> YAIAGNGVRVTYDADGQTITLYRTEGSGLIQMSKPSPLGGPVVGGQEVQDFSHISCDVEQSTSGVMGSGQRMTITSQSMSTGLIRTYVLETSDIEEGVVYTATSYEAGASDVEVSWFIGSVYELYGAEDRIWSYNGGGEGPMHYYDTLQKIDLTDSGKFSRENKQDDTAASIPVSDIYIADGGITVGDASATRREVHTPVQETSDSAQVSIGWPGKVIAAGSVIEIGESFAVVHPGDYYNGLRGYKNAMDHLGVIMPAPGDIPDSSYDLRWESWGWGFNWTIDLIIGKLDELQAAGVKQITLDDGWYTNAGDWALNPEKFPNGASDALRLTDAIHEHGMTALLWWRPCDGGIDSILYQQHPEYFVMDADGRPARLPTPGGGTNPSLGYALCPMADGAIASQVDFVNRAMNDWGFDGFKGDYVWSMPECYNPAHNHASPEESTEKQSEIYRVSYEAMVANDPNVFNLLCNCGTPQDYYSLPYMTQIATADPTSVDQTRRRVKAYKALMGDYFPVTADHNNIWYLSAVGTGSVLIEKRDLSGTAKEEYEKWLGIADTVQLQKGRFIGDLYSYGFDPYETYVVEKDGVMYYAFYKDGSKYSPTGYPDIELKGLDPNKMYRIVDYVNDRVVATNLMGDNAVFNTRFSDYLLVKAVEISEPDP

Recent studies identified two synergistic enzymes from Flavonifractor plautii, namely, N-acetylgalactosamine deacetylase (FpGalNAcDeAc) and galactosaminidase (FpGalNase), which efficiently convert A-type RBCs to O-type by removing A antigens. In this study, we investigated two enzymes from Flavonifractor plautii, N-acetylgalactosamine deacetylase (FpGalNAcDeAc) and galactosaminidase (FpGalNase), which demonstrate synergistic activity in efficiently converting A-type RBCs to O-type. O-type RBCs lack immunodominant sugars found in A (α-N-acetylgalactosamine) and B antigen (galactose), making them essential in emergencies and when matching blood types is not feasible. One promising solution is the enzymatic conversion of all red blood cell (RBC) types into universal O-type RBCs.

We successfully determined the cryo-electron microscopy (cryo-EM) structure of full-length FpGalNase at 2.56 Å resolution. The N-terminal region (residue 27–699) adopts a disc-like conformation divided into three segments: the N-domain, the central GH36 domain, and the C-domain. Structural similarity analysis using the Dali tool revealed that each domain exhibits a structure similar to α-galactosidase, despite low sequence identity. Conserved residues in FpGalNase active site include W317, D346, D347, W387, K461, and D463 (patch A), along with specific non-conserved residues (Y464, C513, and D532) in patch B, which afford a more open catalytic center conformation and may determine its substrate specificity. Site-directed mutagenesis of D463A, Y464A, C513A, and D532A confirmed the functional importance of these residues, as mutations led to significant reductions in conversion activity, with D463A, C513A, and D532A nearly inactive, and the mutants were unable to convert A-type RBCs to O-type in samples from healthy donors. Moreover, comparison between the experimental structure and the AlphaFold-predicted structure revealed a significant deviation in the region from D559 to W564 in the catalytic pocket, highlighting the critical role of experimental data in refining structural models. Sequencing analysis of FpGalNAcDeAc and FpGalNase revealed three mutations in each protein, including V284A in FpGalNAcDeAc and P566L in FpGalNase, located within their catalytic domains. The resolved structures of FpGalNase revealed unique active centers.> MRRAKLAKEKAEKER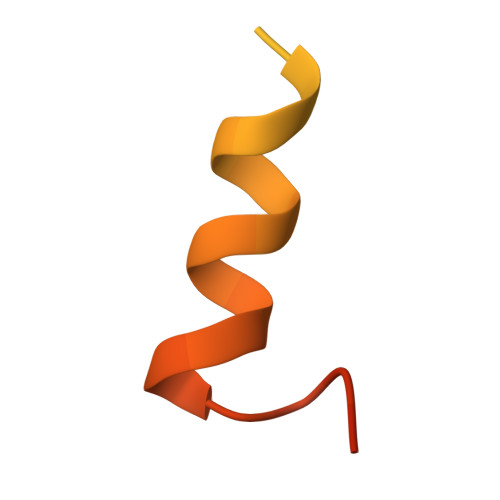LEKQQKREQLIDMNAEGDETGVMDSLLEALQSGAAFRRKRG>HCDLPCGVYDPAQARIEAESVKAIQEKMAANDDLHFQIRATVIKEQRAELAKHHLDVLWSDYFKPPHFESYPELHTLVNEAVKALSAAKASTDPATGQKALDYIAQIDKIFWETKKA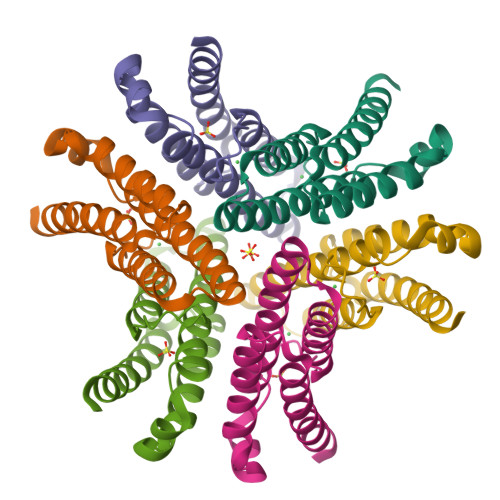[12x]> SMKAIVVINLVKINKKIIPDKIYVYRLFNDPEEELQKEGYSIYRLAYENVGIVIDPENLIIATTKELEYEGEFIPEGEISFSELRNDYQSKLVLRLLKENGIGEYELSKLLRKFRKPKTFGDYKVIPSVEMSVIKHDEDFYLVIHIIHQIQSMKTLWELVNKDPKELEEFLMTHKENLMLKDIASPLKTVYKPCFEEYTKKPKLDHNQEIVKYWYNYHIERYWNTPEAKLEFYRKFGQVDLKQPAILAKFASKIKKNKNYKIYLLPQLVVPTYNAEQLESDVAKEILEYTKLMPEERKELLENILAEVDSDIIDKSLSEIEVEKIAQELENKIRVRDDKGNSVPISQLN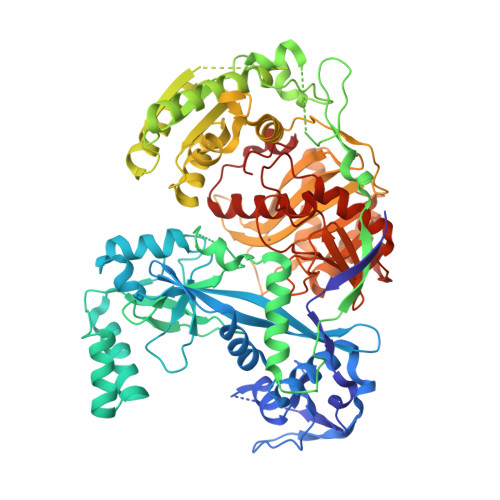VQKSQLLLWTNYSRKYPVILPYEVPEKFRKIREIPMFIILDSGLLADIQNFATNEFRELVKSMYYSLAKKYNSLAKKARSTNEIGLPFLDFRGKEKVITEDLNSDKGIIEVVEQVSSFMKGKELGLAFIAARNKLSSEKFEEIKRRLFNLNVISQVVNEDTLKNKRDKYDRNRLDLFVRHNLLFQVLSKLGVKYYVLDYRFNYDYIIGIDVAPMKRSEGYIGGSAVMFDSQGYIRKIVPIKIGEQRGESVDMNEFFKEMVDKFKEFNIKLDNKKILLLRDGRITNNEEEGLKYISEMFDIEVVTMDVIKNHPVRAFANMKMYFNLGGAIYLIPHKLKQAKGTPIPIKLAKKRIIKNGKVEKQSITRQDVLDIFILTRLNYGSISADMRLPAPVHYAHKFANAIRNEWKIKEEFLAEGFLYFV>[9x]NISPGAEPLILNLSSNIYSSDITQQIEVMRWNFFEESGIPLPKIIVNPVKNNDSAIEFLLYQESIYKDTLIDDTVYFE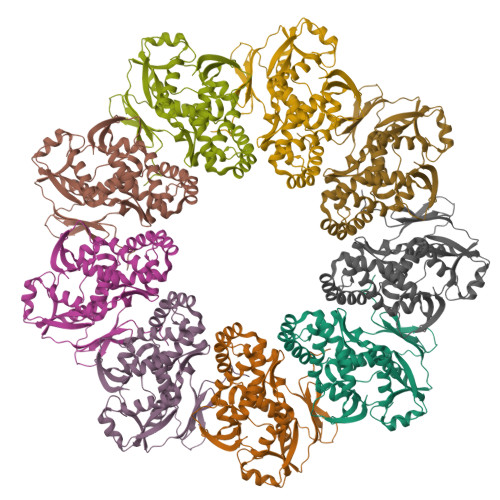AGHAEISFEFVQEKLSTNSIVYKTNKTNQQLAHLTGMDVYATTNDKITFLLKKLVLSNAKEFIGVQETRYLMDIMERKYNELVKELQRQLGLSKIVDILQRLVEENVSIRDLRTIFETLIFWSTKEKDVVILCEYVRIALRRHILGRYSVSGTLLNVWLIGSDIENELRESIRQTSSGSYLNISPERTEQIIGFLKNIMNPTGNGVILTALDIRRYVKKMIEGSFPSVPVLSFQEVGNNIELKVLGTVNDFRA> RPE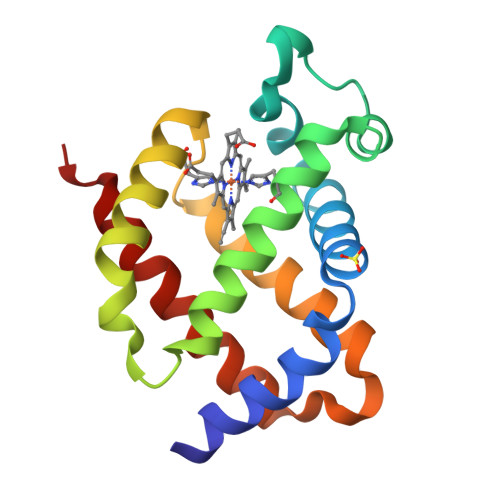SELIRQSWRVVSRSPLEHGTVLFARLFALEPSLLPLFQYNGRQFSSPEDSLSSPEFLDHIRKVMLVIDAAVTNVEDLSSLEEYLTSLGRKHRAVGVRLSSWSTVGESLLYMLEKSLGPDFTPATRTAWSRLYGAVVQAMSRGWDG>[3x]MTDSQQSKPKHVMMMAAGTGGHVFPALAVAKQLQQQGCQVSWLATPTGMENRLLKDQNIPIYQIDIQGVRGNGVIRKLAAPFKILKATFSAMRYMKQLKVDAVAGFGGYVAGPGGLAARLLG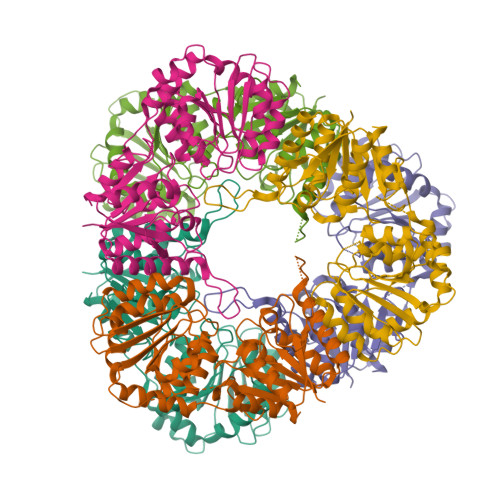IPVLIHEQNAVAGFTNAQLSRVAKVVCEAFPNTFPASEKVVTTGNPVRREITDILSPKWRYDEREQADKPLNILIVGGSLGAKALNERLPPALKQLEVPLNIFHQCGQQQVEATQALYADAPANLTIQVLPFIEDMAKAYSEADLIICRAGALTVTEVATAGVAAVFVPLPIAVDDHQTANAKFLADIGAAKICQQSTMTPEVLNQLFTTLMNRQLLTEMAVKARQHAQPNATQHVVDLIQKM CANALINE | C4 H10 N2 O3 | 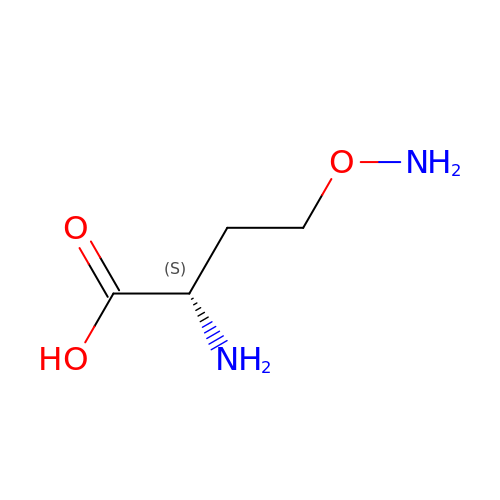FQPGMQABJNQLLF-VKHMYHEASA-N> TNKYHEKWISKFAPGNELSKKYLAKVKERHELKEFNNSISAQDNYAKWTKNNRKLDSLDKEINNLKDEIQSENKAFQ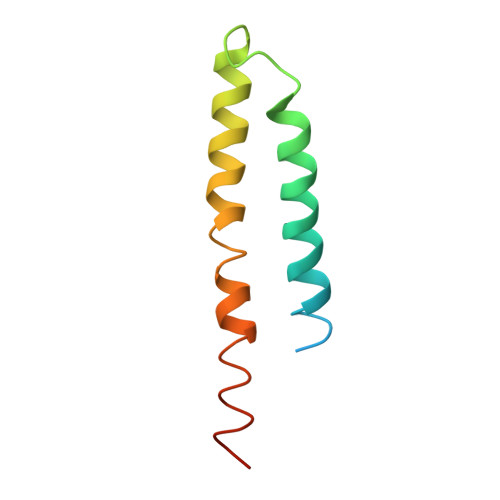AHLHKLR> EFLADSSAHLDLRNFYQLRDYRQHDAPQSQAGNWSQGFVLRLQSGFTGGPLGFGLDATGLLGVKLDSGRGRSNDGTLPFGANSKEPVDDYSHLGLTAKLRYSQTQLQVGILMPQLPVAFRDDVRLLPQTFDGALLTSSEIEGLTLTAGQLWKSRTRESAGSDDMYIMGRDKAHASDEFNLAGATYAFTPRLSASYYYGQLKDIYRQHYLGLLHTLPLGEGLSLRSDLRYFDSGEDGAAISGPVDNRNLNAMLTLRAGAHAFGIGVQKMIGNDAFPVLNGYTTPYVANLMAYQTFTRPQEKSWQLRYDYDFAGLGLPGLNLMTRYVQGRDIDRGAGRADDSEWERNTDLSYVIQSGPLKSVALKWRNITYRSRYGADLDENRF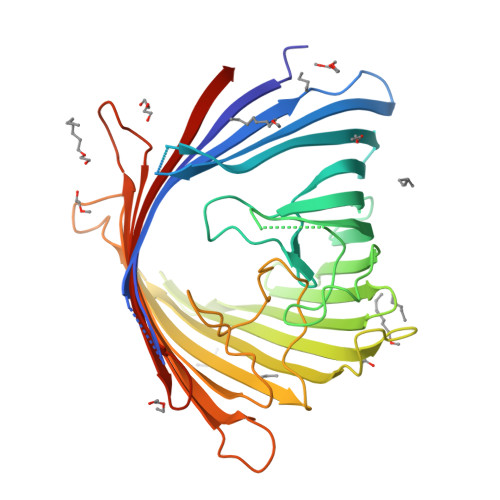IVNYTLKLWGGHHHHHH4'-HYDROXY-7-METHOXYISOFLAVONE | C16 H12 O4 | 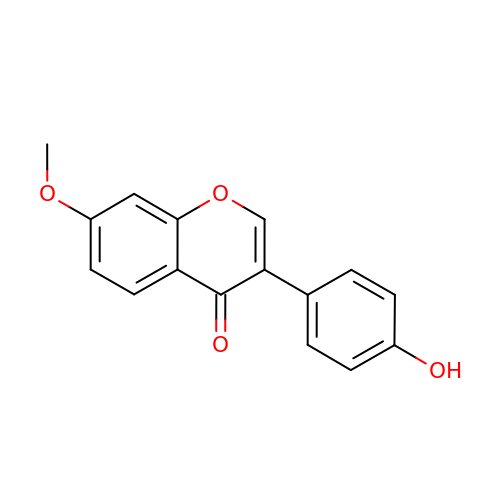LNIQZRIHAMVRJA-UHFFFAOYSA-N> MSLMRDITPDLCDKYESQVTLLNLPLQNFGQRSAFWGEIVTVRCYHDNSKVRDVLSQNGKGKVLVVDGHGSCHKALMGDQLAILAIKNDW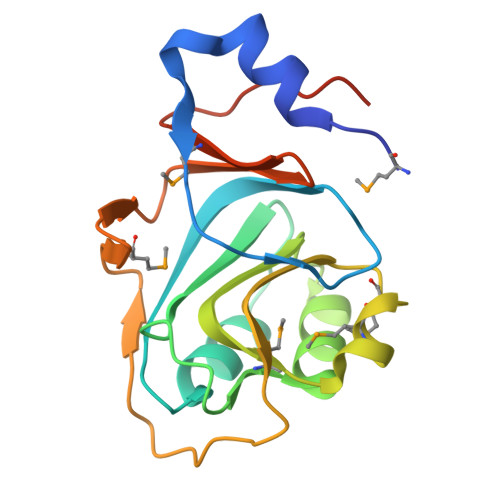EGVIIYGAVRDVVAMSEMDLGIKALGTSPFKTEKRGAGQVNVTLTMQNQIVEPGDYLYADWNGILMSETALDVAEGGSHHHHHH>MISLADLQRRIETGELSPNAAIAQSHAAIEAREKEVHAFVRHDKSARAQASGPLRGIAVGIADIIDTANMPTEMGSEIYRGWQPRSDAPVVMMLKRAGATIIGKTTTTAFASRDPTATLNPHNTGHSPGGSSSGSAAAVGAGMIPLALGTQTGGSVIRPAAYCGTAAIKPSFRMLPTVGVKCYSWALDTVGLFGARAEDLARGLLAMTGRSEFSGIVPAKAPRIGVVRQEFAGAVEPAAEQGLQAAIKAAERAGASVQAIDLPEAVHEAWRIHPIIQDFEAHRALAWEFSEHH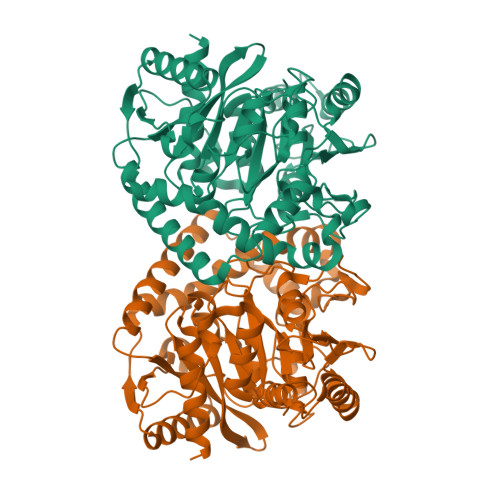DEIAPMLRASLDATVGLTPKEYDEARRIGRRGRRELGEVFEGVDVLLTYSAPGTAPAKALASTGDPRYNRLWTLMGNPCVNVPVLKVGGLPIGVQVIARFGNDAHALATAWFLEDALAKSG[2x]> MFDIGVNLTSSQFAKDRDDVVACAFDAGVNGLLITGTNLRESQQAQKLARQYSSCWSTAGVHPHDSSQWQAATEEAIIELAAQPEVVAIGECGLDFNRNFSTPEEQERA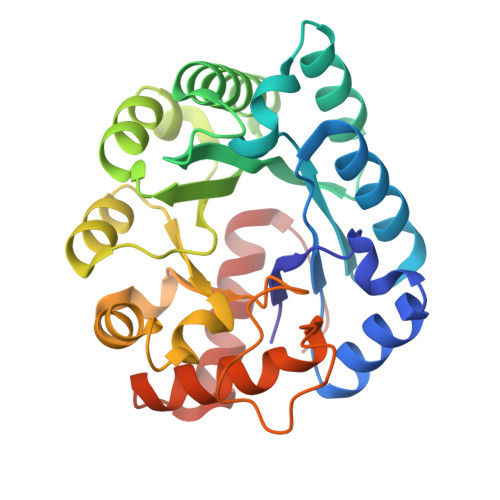FVAQLRIAADLNMPVFMHCRDAHERFMTLLEPWLDKLPGAVLHCFTGTREEMQACVAHGIYIGITGWVCDERRGLELRELLPLIPAEKLLIETDAPYLLPRDLTPKPSSRRNEPAHLPHILQRIAHWRGEDAAWLAATTDANVKTLFGIAFLE> IVGGEDAKPGQFPWQVVLNGKVDAFCGGSIVNEKWIVTA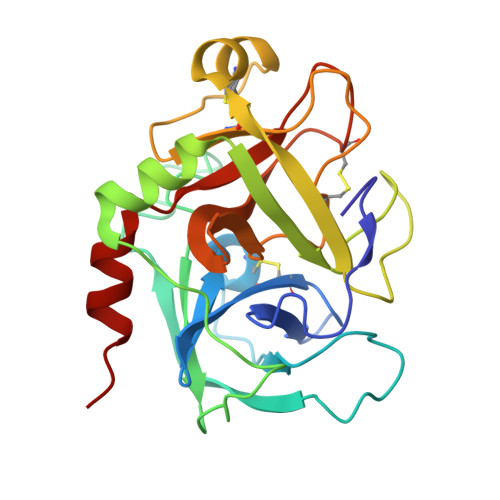AHCVETGVKITVVAGEHNIEETEHTEQKRNVIRIIPHHNYNAAINTYNHDIALLELDEPLVLNSYVTPICIADKEYTNIFLKFGSGYVSGWGRVFHKGRSALVLQYLRVPLVDRATCLRSTKFTITNNMFCAGFHEGGRDSCQGDSGGPHVTEVEGTSFLTGVISWGEECAMKGKYGIYTKVSRYVNWIKEKTKLT>[10x]TRDQNGTWEMESNENFEGYMKALDIDFATRKIAV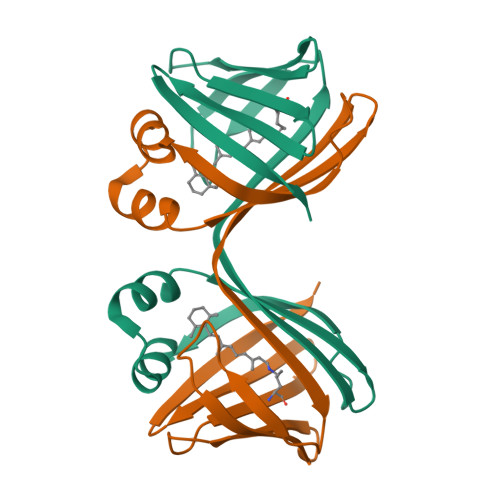RLTQTDVIDQDGDNFKTKTTSTFRNYDVDFTVGVEFDEYTKSLDNRHVKALVTWEGDVLVCVQKGEKENRGWKKWIEGDKLYLELTCGDQVCRQVFKKK;>[2x]TRDQNGTWEMESNENFEGYMKALDIDFATRKIAVRLTQTKVIDQDGDNFKTKTTSTFRNYDVDFTVGVEFDEYTKSLDNRHVKALVTWEGDVLVCVQKGEKENRGWKKWIEGDKLYLELTCGDQVCRQVFKKK> GMDIMLNTADISAAAILLPVEGAQLSELRQIPAEGGPVLHMLRLDSPQFSQFGEIYFSEVLPRRVKAWKRHSLMTQLFAVPVGCIHVVLYDGREKSPTSGRLAQVTLGRPDNYRLLRIPPQVWYGFAATGDTPALVANCTDI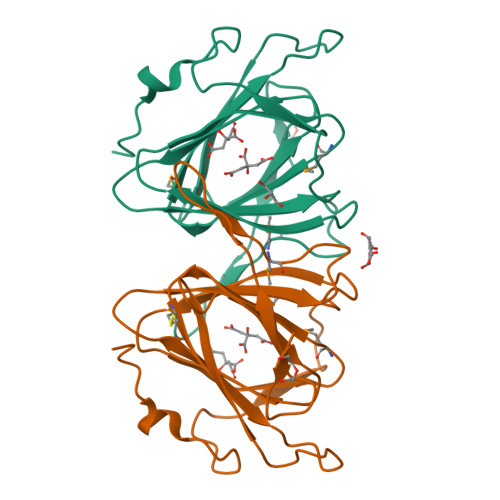PHRQGESERAPQDAPFIPFSWAGADLSGTPVM> SHMTNLQTFELPTEVTGCAADISLGRALIQAWQKDGIFQIKTDSEQDRKTQEAMAASKQFCKEPLTFKSSCVSDLTYSGYVASGEEVTAGKPDFPEIFTVCKDLSVGDQRVKAGWPCHGPVPWPNNTYQKSMKTFMEELGLAGERLLKLTALGFELPINTFTDLTRDGWHHMRVLRFPPQTSTLSRGIGAHTDYGLLVIAAQDDVGGLYIRPPVEGEKRNRNWLPGESSAGMFEHDEPWTFVTPTPGVWTVFPGDILQFMTGGQLLSTPHKVKLNTRERFACAYFHEPNFEASAYPLFEPSANERIHAGEHFTNMFMRCYPDRITTQRINK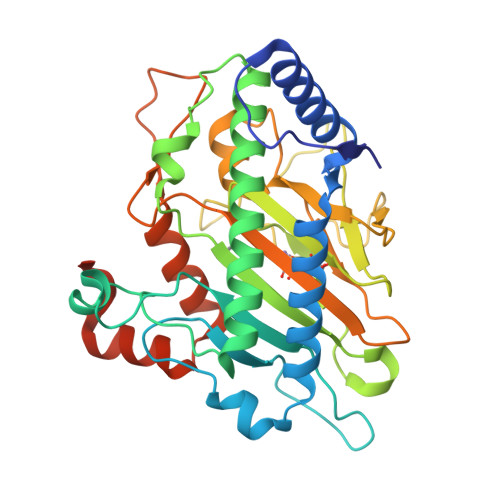ENRLAHLEDLKKYSDTRATGS>[4x]MAPVLSKDVADIESILALNPRTQSHAALHSTLAKKLDKKHWKRNPDKNCFHCEKLENNFDDIKHTTLGERGALREAMRCLKCADAPCQKSCPTHLDIKSFITSISNKNYYGAAKMIFSDNPLGLTCGMVCPTSDLCVGGCNLYATEEGSINIGGLQQFASEVFKAMNIPQ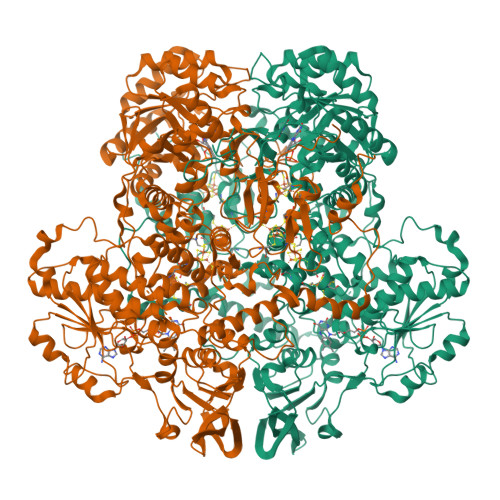IRNPCLPSQEKMPEAYSAKIALLGAGPASISCASFLARLGYSDITIFEKQEYVGGLSTSEIPQFRLPYDVVNFEIELMKDLGVKIICGKSLSENEITLNTLKEEGYKAAFIGIGLPEPKTDDIFQGLTQDQGFYTSKDFLPLVAKSSKAGMCACHSPLPSIRGAVIVLGAGDTAFDCATSALRCGARRVFLVFRKGFVNIRAVPEEVELAKEEKCEFLPFLSPRKVIVKGGRIVAVQFVRTEQDETGKWNEDEDQIVHLKADVVISAFGSVLRDPKVKEALSPIKFNRWDLPEVDPETMQTSEPWVFAGGDIVGMANTTVESVNDGKQASWYIHKYIQAQYGASVSAKPELPLFYTPVDLVDISVEMAGLKFINPFGLASAAPTTSSSMIRRAFEAGWGFALTKTFSLDKDIVTNVSPRIVRGTTSGPMYGPGQSSFLNIELISEKTAAYWCQSVTELKADFPDNIVIASIMCSYNKNDWMELSRKAEASGADALELNLSCPHGMGERGMGLACGQDPELVRNICRWVRQAVQIPFFAKLTPNVTDIVSIARAAKEGGADGVTATNTVSGLMGLKADGTPWPAVGAGKRTTYGGVSGTAIRPIALRAVTTIARALPGFPILATGGIDSAESGLQFLHSGASVLQVCSAVQNQDFTVIQDYCTGLKALLYLKSIEELQGWDGQSPGTESHQKGKPVPRIAELMGKKLPNFGPYLEQRKKIIAEEKMRLKEQNAAFPPLERKPFIPKKPIPAIKDVIGKALQYLGTFGELSNIEQVVAVIDEEMCINCGKCYMTCNDSGYQAIQFDPETHLPTVTDTCTGCTLCLSVCPIIDCIRMVSRTTPYEPKRGLPLAVNPVC FdlA from Flavobacterium sp. SA-0082 is an endo-type fucoidan-degrading enzyme that cleaves the sulfated fuco-glucuronomannan (SFGM) through a lytic mechanism. We show that the FdlA-NTD adopts a right-handed parallel β-helix fold, and possesses a substrate binding site composed of a long groove and a unique alkaline pocket. Our structural, biochemical, and enzymological analyses strongly suggest that FdlA-NTD utilizes catalytic residues different from other β-helix polysaccharide lyases, potentially representing a novel polysaccharide lyase family. Here, we report crystal structures and enzymological characterization of wild type (WT) and eight single mutants of the catalytic N-terminal domain (NTD) of FdlA, revealing its unique substrate binding pocket and identifying the key catalytic residues.

We first measured the enzymatic activity of 12 mutants and found that eight of them (D137A, K141A, H176A, F179A, E236A, R240A, Y242A, and Y242F) almost completely abolished their activities, H279A mutant retained approximately 65% of the activity compared with WT, while mutations of Asn243, Arg272, and Tyr322 to Ala only negligibly affect their activities. Residue His176 is located close to Tyr242, and the H176A mutation shows a slight influence on the Tyr242 side chain conformation. Therefore, mutation of Phe179 and His176 possibly results in the dysfunction of Tyr242 and hence loss of the catalytic activity of FdlA-NTD. In addition, His176 forms a hydrogen bond (2.8 Å) with the hydroxyl group of Tyr242 side chain in WT, implying another possibility that it might play a role in providing a proton to Tyr242 to facilitate the catalytic reaction. Based on our structural and docking models, several positively charged residues such as Arg240, His176, and Lys141, located near the +1 subsite, potentially serve as neutralizers in FdlA-NTD, weakening the negative charge of the C-5 carboxyl group at +1 subsite, and making the C-5 proton susceptible to the attack by a Brønsted base. Next, the positively charged residues including Arg240 and His176, which are located near the +1 subsite, neutralize the C-5 carboxyl group of D-GlcUA at +1 subsite, thus reducing the pKa of the C-5 proton, making it more susceptible to the attack by a base.

>[2x]HHHHHHSSGLVPRGSHMQTTTVYSLEDLLPYLKQDNVDVKLAPGTYNVNGFDVGEDRLFSTTPLFLFEGSNSTYDFTDVKLNINTVVLTKFGNNEVNEIQILGNNNVLKNLKLEDIGTTAPSNRAQSIVIDGRDNRIEGFHLTIRGSYPYGYGDAFGKGGGSVINHRKHSGVLIRGLRNHLKDCTIISRSYGAIVFMQAASYPTVEGCYIEGEMRSTDDMLAEEGTGSPADKVDFMTVWGYKLPAGYMMSLQEGGIRAYNAGTTYIDGVEIQRATDNPTVLNCTIKNARTGVTLAHANGTKYVEGCTVLGCENGYSIGSGTVVNCGADAIYGPVFKNTYGSDKGYNADITILPPSDAYYNGHDAVAYIGGSNHNLTFRSEITEIPSNLKIMVSGDLQGLRVLHGSNPSQNNFAGTNIVLRNLTNFPVDLHSDSSNITVTSCDTDNITDNGTNNSIEAIDCDSD> GSHMANPLAPYTLPQIATKVQVKHVPGKGRCLYTKHDLEPGSIIFVETPVLVAIPSLDEELWSVLTEINDEEALELPPVWHLAAICSLTMLDDEKKKICLDKWVPDPDRAPSDDVLRVINRAGLQVHPKLYERMLMVWRYNSFGHHTEQHGLVLYNRISMMAHSCRATACWHYGEDDAFILRARVKLQAGDELTISYIGDDDLFKSTNVRREKVYGWLFTCQCVRCAAPVDNARGFRCPLCGTGAMFFKTEDGETTSSACTICQAFPTQET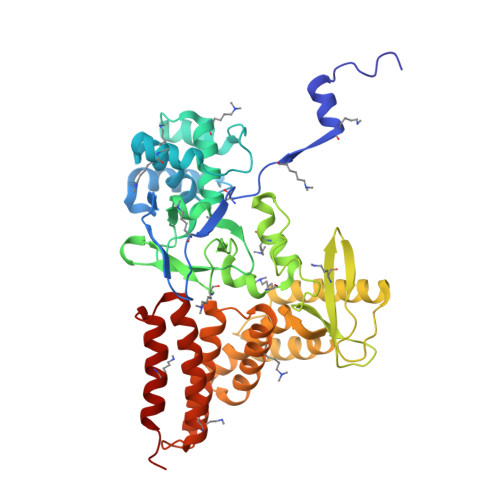IQEYLDFEQAYVDRLAETDKSDVPDAELVYNQATRVFAQHWVLYQLHTILFEGYRDAGNSESASFHQMERIKYVSQVMPLASYTLAWLYEEMGDTMLNKAEESGPEVPAHKLNVISRHFEDAYNLLYILCGEDHDYTVAAGTKKTACEERLPAS>MRVLLIHSDYIEYEVKDKALKNPEPISEDMKRGRMEEVLVAFISVEKVDEKNPEEVSLKAIEEISKVAEQVKAENVFVYPFAHLSSELAKPSVAMDILNRVYQGLKERGFNVGKAPFGYYKAFKISCKGHPLAELSRTIVPEEARVE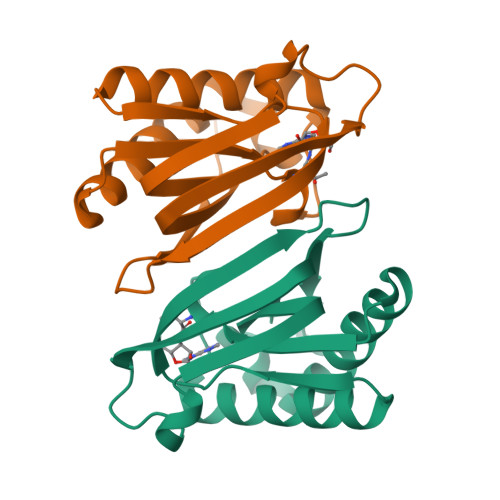[2x]> SHMASAEHSFDVNEVIKDFPILDQKVNGKRLAYLDSTATSQTPVQVLNVLEDYYKRYNSNVHRGVHTLGSLATDGYENARETVRRFINAKYFEEIIFTRGTTASINLVAHSYGDANVEEGDEIVVTEMEHHANIVPWQQLAKRKNATLKFIPMTADGELNIEDIKQTINDKTKIVAIAHISNVLGTINDVKTIAEIAHQHGAIISVDGAQAAPHMKLDMQEMNADFYSFSGHKMLGPTGIGVLFGKRELLQKMEPIEFGGDMIDFVSKYDATWADLPTKFEAGTPLIAQAIGLAEAIRYLERIGFDAIHKYEQELTIYAYEQMSAIEGIEIYGPPKDRRAGVITFNLQDVHPHDVATAVDTEGVAVRAGHHCAQPLMKWLNVSSTARASFY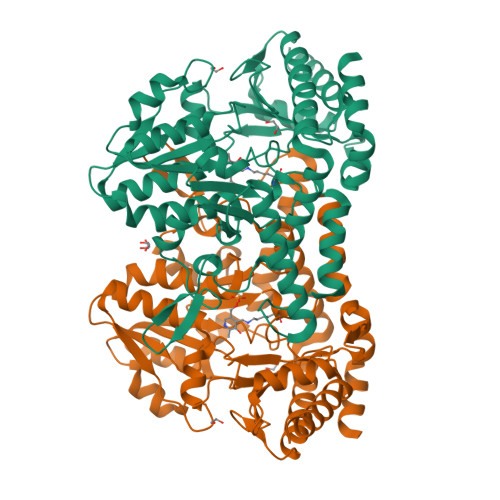IYNTKEDVDQLINALKQTKEFFS>[2x]SNAMSDIKHAKLLILGSGPAGYTAAIYAARANLKPVLVTGLQQGGQLTTTDEIENWPGDFEMTTGSGLMQRMLQHAEKFETEIVFDHINRVDLSSRPFKLFGDVQNFTCDALIIATGASARYIGLPSEENYKGRGVSACATCDGFFYRNKPVGVIGGGNTAVEEALYLANIASTVHLIHRRDSFRAEKILIDR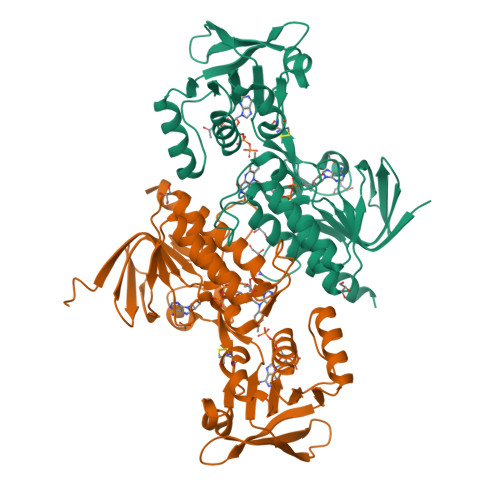LYKKVEEGKIVLHTDRTLDEVLGDNMGVTGLRLANTKTGEKEELKLDGLFVAIGHSPNTEIFQGQLELNNGYIVVKSGLDGNATATSVEGVFAAGDVMDHNYRQAITSAGTGCMAALDAERYLDAQEA>[2x]MSQAATPAADGKVKISIDPLTRVEGHLKIEVEVKDGKVVDAKCSGGMFRGFEQILRGRDPRDSSQIVQRICGVCPTAHCTASVMAQDDAFGVKVTTNGRITRNLIFGANYLQSHILHFYHLAALDYVKGPDVSPFVPRYANADLLTDRIKDGAKADATNTYGLNQYLKALEIRRICHEMVAMFGGRMPHVQGMVVGGATEIPTADKVAEYAARFKEVQKFVIEEYLPLIYTLGSVYTDLFETGIGWKNVIAFGVFPEDDDYKTFLLKPGVYIDGKDEEFDSKLVKEYVGHSFFDHSAPGGLHYSVGETNPNPDKPGAYSFVKAPRYKDKPCEVGPLARMWVQNPE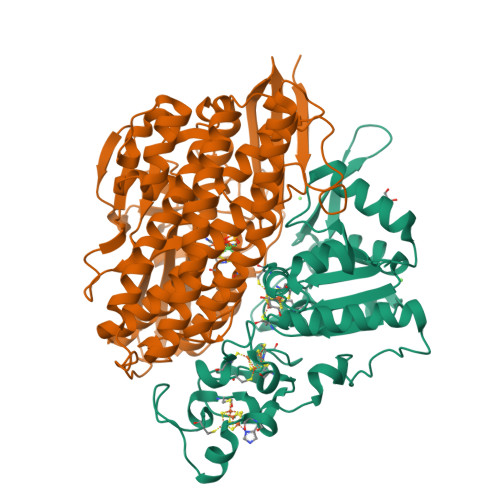LSPVGQKLLKELYGIEAKNFRDLGDKAFSIMGRHVARAEETWLTAVAVEKWLKQVQPGAETYVKSEIPDAAEGTGFTEAPRGALLHYLKIKDKKIENYQIVSATLWNANPRDDMGQRGPIEEALIGVPVPDIKNPVNVGRLVRSYDPULGCAVH;>MTEGAKKAPVIWVQGQGCTGCSVSLLNAVHPRIKEILLDVISLEFHPTVMASEGEMALAHMYEIAEKFNGNFFLLVEGAIPTAKEGRYCIVGETLDAKGHHHEVTMMELIRDLAPKSLATVAVGTCSAYGGIPAAEGNVTGSKSVRDFFADEKIEKLLVNVPGCPPHPDWMVGTLVAAWSHVLNPTEHPLPELDDDGRPLLFFGDNIHENCPYLDKYDNSEFAETFTKPGCKAELGCKGPSTYADCAKRRWNNGINWCVENAVCIGCVEPDFPDGKSPFYVAE[2x]>GRQRKNEALAPPLLDAEPARGAGGRGGDHPSVAVGIRRVSNVSAASLVPAVPQPEADNLTLRYRSLVYQLNFDQTLRNVDKAGTWAPRELVLVVQVHNRPEYLRLLLDSLRKAQGIDNVLVIFSHDFWSTEINQLIAGVNFCPVLQVFFPFSIQLYPNEFPGSDPRDCPRDLPKNAALKLGCINAEYPDSFGHYREAKFSQTKHHWWWKLHFVWERVKILRDYAGLILFLEEDHYLAPDFYHVFKKMWKLKQQECPECDVLSLGTYSASRSFYGMADKVDVKTWKSTEHNMGLALTRNAYQKLIECTDTFCTYDDYNWDWTLQYLTVSCLPKFWKVLVPQIPRIFHAGDCGMHHKKTCRPSTQSAQIESLLNNNKQYMFPETLTISEKFTVVAISPPRKNGGWGDIRDHELCKSYRR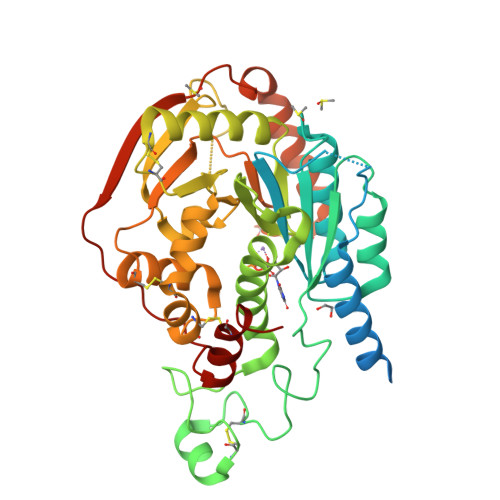LQ[2x]4-(naphthalen-1-yl)-1H-indole-2-carboxylic acid | C19 H13 N O2 | 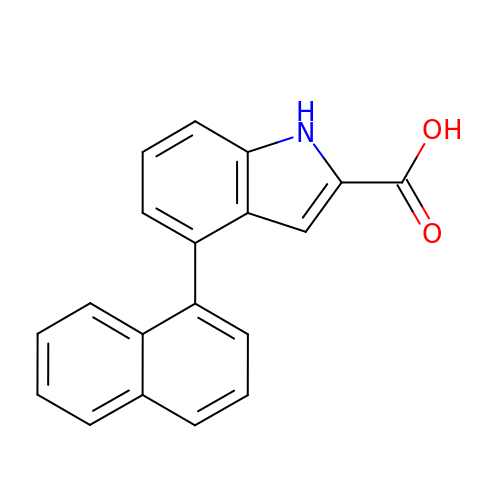QVAVQSOUZBBMKK-UHFFFAOYSA-N1H-imidazol-2-amine 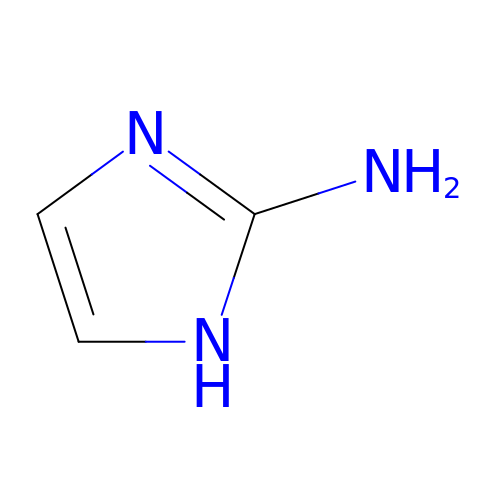| C3 H5 N3 | DEPDDPLQZYCHOH-UHFFFAOYSA-N N-(10-aminodecanoyl)-L-seryl-N-(2-cyclohexylethyl)-L-lysinamide | C27 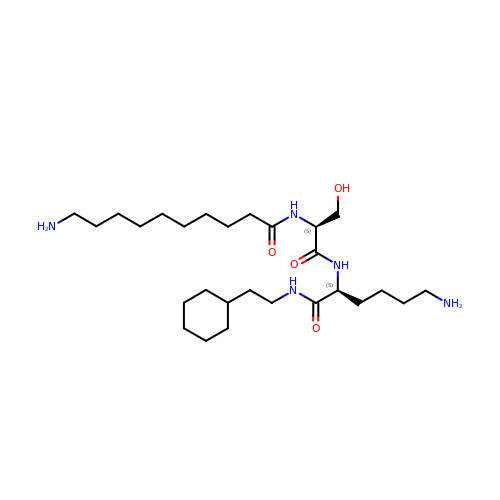H53 N5 O4 | OVRFOVZVAWIPDE-ZEQRLZLVSA-N> YYFEPNTAIGANGYKIID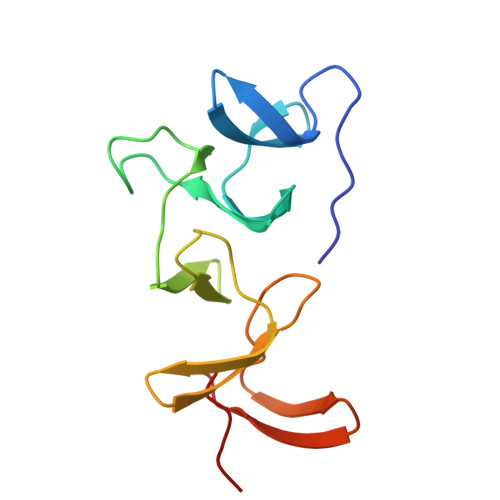NKNFYFRNGLPQIGVFKGPNGFEYFAPANTDANNIEGQAIRYQNRFLHLLGNIYYFGNNSKAVTGWQTINGNMYYFMPDTAMAAAGGLFEIDGVIYFFGVDGVKAPGIY> MRSNSQGLSLTDSVYERLLSERIIFLGSEVNDEIANRLCAQILLLAAEDASKDISLYINSPGGSISAGMAIYDTMVLAPCDIATYAMGMAASMGEFLLAAG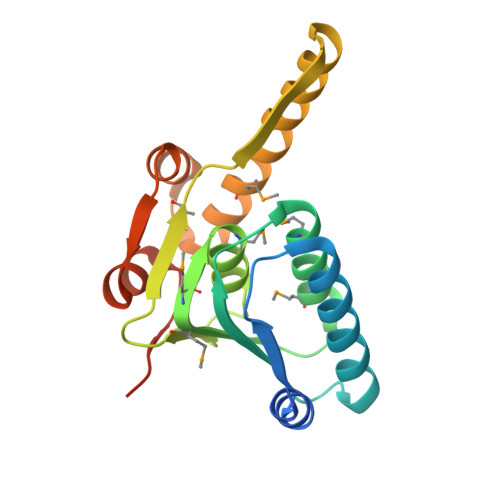TKGKRYALPHARILMHQPLGGVTGSAADIAIQAEQFAVIKKEMFRLNAEFTGQPIERIEADSDRDRWFTAAEALEYGFVDHIITRAHVNGEAQ>GSH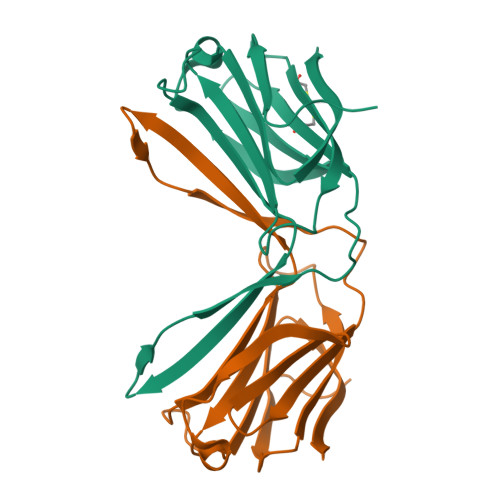MSSLPVPYTLPVSLPVGSCVIITGTPILTFVKDPQLEVNFYTGMDEDSDIAFQFRLHFGHPAIMNSCVFGIWRYEEKCYYLPFEDGKPFELCIYVRHKEYKVMVNGQRIYNFAHRFPPASVKMLQVFRDISLTRVLISD[2x]>[3x]CGIVGAIAQRDVAEILLEGLRRLEYRGYDSAGLAVVDAEGHMTRLRRLGKVQMLAQAAEEHPLHGGTGIAHTRWATHGEPSEVNAHPHVSEHIVVVHNGIIENHEPLREELKARGYTFVSETDTEVIAHLVNWELKQGGTLREAVLRAIPQLRGAYGTVIMDSRHPDTLLAARSGSPLVIGLGMGENFIASDQLALLPVTRRFIFLEEGDIAEITRRSVNIFDKTGAEVKRQDIESNLQYDAGDKGIYRHYMQKEIYEQPNAIKNTLTGRISHGQVDLSELGPNADELLSKVEHIQILACGTSYNSGMVSRYWFESLAGIPCDV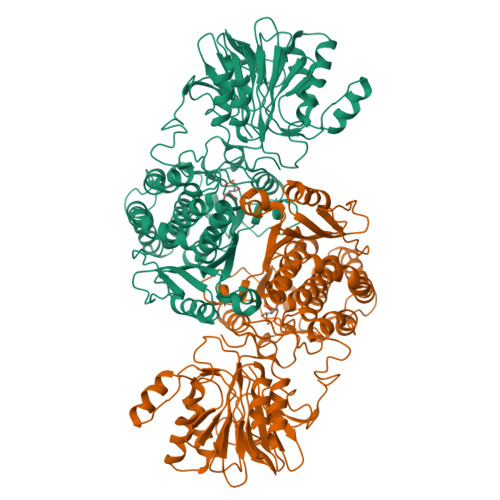EIASEFRYRKSAVRRNSLMITLSQSGETADTLAGLRLSKELGYLGSLAICNVPGSSLVRESDLALMTNAGTEIGVASTKAFTTQLTVLLMLVAKLSKLKGLDASIEHDIVHGLQALPSRIEQMLSQDKRIEALAEDFSDKHHALFLGRGDQYPIALEGALKLKEISYIHAEAYAAGELKHGPLALIDADMPVIVVAPNNELLEKLKSNIEEVRARGGQLYVFADQDAGFVSSDNMHIIEMPHVEEVIAPIFYTVPLQLLAYHVALIKGTDVDQPRNLAKSVTVE>[3x]GSAKDPHNHYIWAKLSAYHIAELLEQEKRYDESLAIIEEARVIWPNVPEFPLKKANILYVNHQLEDAKEIYQSLLENAAIDYQPIVLYEATNFMPHKMLGTIYLEEKDYTRAMTHFSKAYAENSSDYGVMFQMIMLLSKFHQPKEIFAFMERHHFISSTETGLRLLSMTTQQGYAELSELIVQSLTDVYPPVAEATEVKIATIRNVFPVISESAILFGIKEELIDAADLCLWHYENPQLPIENVMKNSDVGDIYDFIFENGPRISKKRYLFVLERAIALGKGEFADYLLALRNVYHDSINSHIADLFFQYDFADIALDFYNIVDADEVTKQGYINLINYLVDADVLDEALAIAERGIDNFSTDFRFYLWAIKIDTENRANRISEAMDEFPNNRYLAKLLDEVTMLQDTVTNNR;>[3x]GSAKDPMPKSEIRKLLQEIKKQVDNPGNSSTTEIKKMASEAGIDEQTAEEIYHLLTEFYQAVEEHGGIEKYMHSNISWLKIELELLSACYQIAILEDMKVLDISEMLSLNDLRIFPKTPSQLQNTYYKLKKELIQVEDIPKNKPGRKRKTQKNTKKEKTNIFGKVVPA

Listeria monocytogenes GmaR is a thermosensor protein that coordinates flagellar expression by binding the master transcriptional repressor of flagellar genes (MogR) in a temperature-responsive manner. In L. monocytogenes, flagellar expression is transcriptionally coordinated in a temperature-dependent manner by the motility gene repressor MogR and the antirepressor GmaR. GmaR forms an intermolecular complex with MogR and prevents MogR from binding to operator DNA, resulting in the derepression of flagellar transcription. GmaR is a four-domain protein that consists of glycosyltransferase, TPR, linker and antirepressor domains.

To visualize the GmaR–MogR interaction that is required for derepression of flagellar expression, a GmaR–MogR complex structure was determined by X-ray crystallography using the MogRD protein and an N-terminally truncated GmaR protein (GmaR231-637) that contains residues 231–637. In the GmaR–MogR complex, one polypeptide chain of GmaR interacts with one MogR chain, consistent with the 1:1 molar ratio observed by native PAGE and gel-filtration chromatography. The asymmetric unit of the GmaR–MogR crystal contains three copies of the 1:1 complex, which exhibit similar quaternary structures. MogR-bound GmaR (GmaRMogR) adopts a duck swim ring-like circular structure consisting of three α-helical domains, similar to the GmaRApo structure, with a root-mean-square deviation value of 1.27 Å (393 Cα atoms). In the GmaR–MogR complex structure, the intermolecular interaction between GmaR and MogR occurs in two spatially separated regions, antirepressive sites 1 and 2 (buried surface areas of ∼350 and ∼540 Å2, respectively). Antirepressive sites 1 and 2 are observed in the C-terminal extension and main body of MogR, respectively. At antirepressive site 1, a small cavity in GmaR on the convex side in the middle of the antirepressor domain accommodates MogR residues 152–156 and 160 from the C-terminal coil structure. The hydrophobic side chains of the MogR I155 and F156 residues at the protrusion of the C-terminal coil structure are embedded into the hydrophobic cavity of GmaR. In the GmaR–MogR structure, GmaR residues from the α26 and α27 helices and their connecting loop make contacts with MogR main body residues at the H6 and H7 helices. In the overlaid GmaR–MogR and MogR–dsDNA structures, site 1-adjacent GmaR residues substantially clash with dsDNA atoms at the MIG site, suggesting that the site 1 interaction limits the accessibility of dsDNA to the MIG site of MogR via a spatial restraint.> SNANEAQQYYLDADEAEAWIGEQELYVISDEIPKDEEGAIVMLKRHLRQQRAVEDYGRNIKQLASRAQGLLSAGHPEGEQIIRLQGQVDKHYAGLKDVA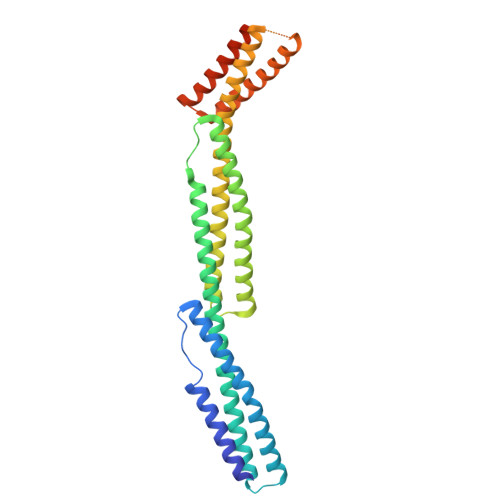EERKRKLENMYHLFQLKRETDDLEQWISEKELVASSPEMGQDFDHVTLLRDKFRDFARETGAIGQERVDNVNAFIERLIDAGHSEAATIAEWKDGLNEMWADLLELIDTRMQLLAASYDLHRYFYTGAEILGLIDEKHRELPEDVGLDASTAESFHRVHTAFERDVHLLGVQVQQFQDVATRLQTAYAGEKAEAIQNKEQEVSAAWQALLDACAGRRTQLVDTADKF>MHHHHHHMGLNTAIATRVNGTPPPEVPIADIELGSLDFWALDDDVRDGAFATLRREAPISFWPTIELPGFVTGNGHWALTKYDDVFYASRHPDIFSSYPNITINDQTPELAEYFGSMIVLDDPRHQRLRSIVSRAFTPKVVARIEAAVRDRAHRLVSSMIANNPDRQADLVSELAGPLPLQIICDMMGIPKADHQRIFHWTNVILGFGDPDLATDFDEFMQVSADIGAYATALAEDRRVNHHDDLTSSLVEAEVDGERLSSREIASFFILL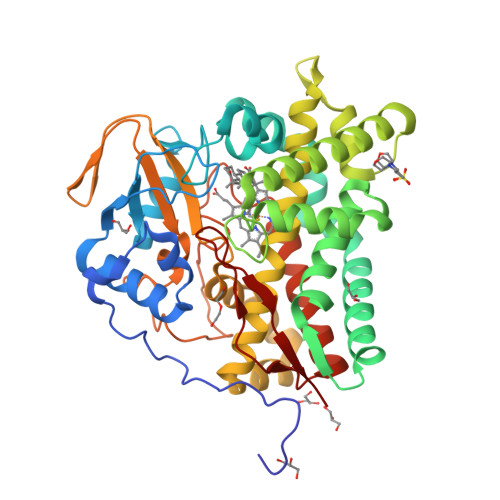VVAGNETTRNAITHGVLALSRYPEQRDRWWSDFDGLAPTAVEEIVRWASPVVYMRRTLTQDIELRGTKMAAGDKVSLWYCSANRDESKFADPWTFDLARNPNPHLGFGGGGAHFCLGANLARREIRVAFDELRRQMPDVVATEEPARLLSQFIHGIKTLPVTWS[4x]> GPLGSALGMAAVTLHLRAETKPLEARAALTPTTVKKLIAKGFKIYVEDSPQSTFNINEYRQAGAIIVPAGSWKTAPRDRIIIGLKEMPETDTFPLVHEHIQFAHCYKDQAGWQNVLMRFIKGHGTLYDLEFLENDQGRRVAAFGFYAGFAGAALGVRDWAFKQTHSDDEDLPAVSPYPNEKALVKDVTKDYKEALATGARKPTVLIIGALGRCGSGAIDLLHKVGIPDANILKWDIKETSRGGPFDEIPQADIFINCIYLSKPIAPFTNMEKLNNPNRRLRTVVDVSADTTNPHNPIPIYTV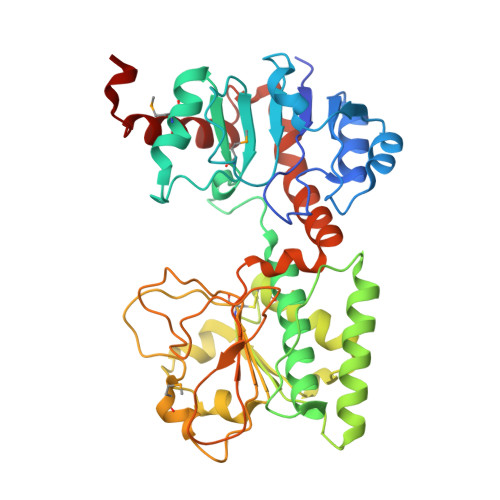ATVFNKPTVLVPTTAGPKLSVISIDHLPSLLPREASEFFSHDLLPSLELLPQRKTAPVWVRAKKLFDRHCARVKRSSRL>AMALEARLEQASILKKVVDAIKDLV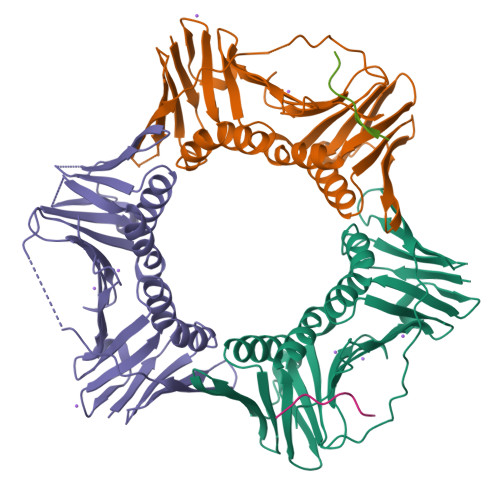QDCNFDCNDSGIALQAMDNSHVALVSMMLKAEGFSPYRCDRNIALGVNLTSLTKVLRAAQNEDILTLKAEDAPDVLNLVFESSETDRISEYDLKLMDIDQEHLGIPETEYAATITMPSNEFKRITTDLMAMSESVTIEANKDGVKFSCQGDIGNGSVTLRQHTNVEKPNESIEIELSEPVSLTFSLKYLVNFCKASALSNTVKICLSNEVPLLVEYSLGGSSYLRFYLAPKIGDDE[6x];>KHQSTLNFKHRVTKP[4x]7,10,13-TRI(CARBOXYMETHYL)-5,15-DIOXO-4,7,10,13,16-PENTAAZA-1,19-DITHIANONADECANE | C18 H33 N5 O8 S2 | 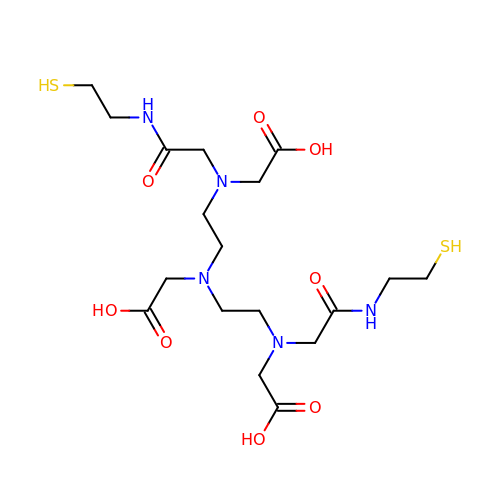MRDWXQKAAKNXSP-UHFFFAOYSA-N> MASKEAHVSLARGEQSVKRIKEFDPG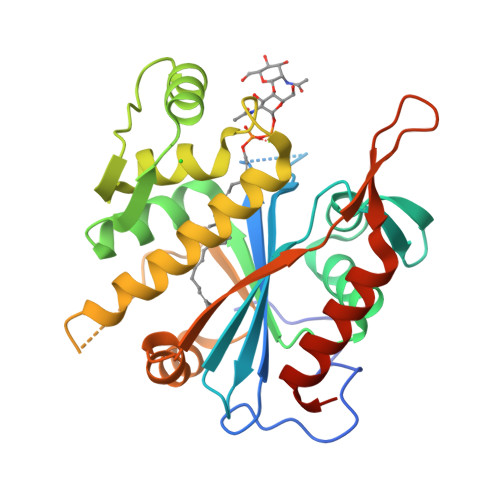KDSFSVLLLGIDAREKNGETVDQARSDANVLVTFNRKEKTAKMLSIPRDAYVNIPGHGYDKFTHAHAYGGVDLTVKTVEEMLDIPVDYVVESNFTAFEDVVNELNGVKVTVKSDKVIQQIKKDTKGKVVLQKGTHTLDGEEALAYVRTRKADSDLLRGQRQMEVLSAIIDKSKSLSSIPAYDDIVDTMGQNLKMNLSLKDAIGLFPFITSLKSVESIQLTGYDYEPAGVYYFKLNQQKLQEVKKELQNDLGVLEHHHHHH>MELFLAGRRVLVTGAGKGIGRGTVQALHATGARVVAVSRTQADLDSLVRECPGIEPVCVDLGDWEATERALGSVGPVDLLVNNAAVALLQPFLEVTKEAFDRSFEVNLRAVIQVSQIVARGLIARGVPGAIVNVSSQCSQRAVTNHSVYCSTKGALDMLTKVMALELGPHKIRVNAVNPTVVMTSMGQATWSDPHKAKTMLNRIPLGKFAEVEHVVNAILFLLSDRSGMTTGSTLP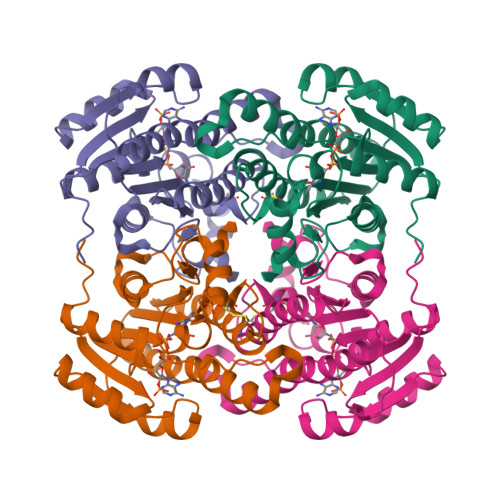VEGGFWAC[2x]Human APOBEC3G (hA3G) is a member of apolipoprotein B mRNA editing enzyme catalytic polypeptide like (APOBEC) family, and is one of the most effective antiviral host restriction factors against exogenous retroviral pathogens such as human immunodeficiency virus type 1 (HIV-1) and endogenous retroviral derived remnants on the human genome. hA3G is a DNA/RNA cytidine deaminase converting 3′ target cytidine (C) in 5′-CC-3′ or 5′-CCC-3′ motif to uridine (U) within single-stranded DNA (ssDNA)9–15 or single-stranded RNA (ssRNA). hA3G has two cytidine deaminase domains in tandem, the N-terminal CD1 (or NTD) and C-terminal CD2 (or CTD). The ability to bind nucleic acids and form oligomerization is attributed mainly to CD1/NTD (referred to as CD1 hereafter), while deaminase activity is performed by CD2/CTD (referred to as CD2 hereafter). In this study, we describe four structures of a soluble primate rA3G variant from rhesus macaque, rA3GR8/E259A, in complex with AA and GA dinucleotide-containing RNA molecules in the form of ssRNA and dsRNA with 5′- or 3′-overhangs.

RNA2-AA was modified with 3′ overhang on both strands (5′ dsRNA8-A9A10U11U12U13U14, designated as RNA2-AAxtal, with dsRNA8 5′-CCCGUGGG-3′/5′-CCCACGGG-3′). Complexes with RNA1-AAxtal and RNA2-AAxtal were determined as two different types of dimers with two rA3G molecules binding to one RNA molecule at 2.90 and 3.10 Å, respectively. In both cases, the electron density maps of RNA were of sufficient quality to allow de novo building of a complete dsRNA8 plus three nucleotides (3-nt) on each AA dinucleotide-containing overhang (5′-U2A3A4-dsRNA8-3′ and 5′-dsRNA8-A9A10U11-3′). In both dimer models, there are no direct contacts between the two rA3GR8/E259A monomers, which is reminiscent of A3H-dsRNA complexes showing RNA-assisted dimer formation. In the 3′-overhang dsRNA co-crystal structure, there are multiple contacts between dsRNA8 and rA3G, resulting in a relatively rigid structure with defined electron density for the dsRNA. The dsRNA8 has a G-C base pair (G8-C1) 5’ to the bound AA ssRNA core (5′-A9A10-3′), with G8 (in the sequence 5′-G8A9A10-3′) making five hydrogen bonds with S28 through its base/sugar moiety (bond lengths 2.5−3.7 Å), including two that are guanine base specific (carbonyl/amyl groups of S28 peptide backbone with N2/N3 groups of G8, respectively). Additional five hydrogen bonds are present between the side chains of R24/N176/N177 and the phosphate backbone of C5, G6, G7, and G8 of the dsRNA (bond lengths 2.8−3.7 Å). Contacts with the phosphate backbone and the base G8 in the dsRNA region enhances the overall stability of the dsRNA8 structure. When in complex with 5′- or 3′-overhang dsRNA containing unpaired AA dinucleotide, RNA-mediated rA3G dimers are formed. These RNA-mediated dimers can have different dimerization arrangements, depending on whether the ssRNA is 5′- or 3′-overhang and the length of the dsRNA region.

>[2x]GPGGSGGMKPQIRNMVEPMDPRTFVSNFNNRPILSGLDTVWLCCEVKTKDPSGPPLDAKIFQGKVYPKAKYHPEMRFLRWFHKWRQLHHDQEYKVTWYVSWSPCTRCANSVATFLAKDPKVTLTIFVARLYYFWKPDYQQALRILAEAGATMKIMNYNEFQDCWNKFVDGRGKPFKPWNNLPKHYTLLQATLGELLRHLMDPGTFTSNFNNKPWVSGQHETYLCYKVERLHNDTWVPLNQHRGFLRNQAPNIHGFPKGRHAALCFLDLIPFWKLDGQQYRVTCFTSWSPCFSCAQEMAKFISNNEHVSLCIFAARIYDDQGRYQEGLRTLHRDGAKIAMMNYSEFEYCWDTFVDRQGRPFQPWDGLDEHSQALSGRLRAILQNQGN>[2x]SNAMIRKYRYGAPFDTEALTEKIETAEEAFPYGEISQKEGFAFTYIMDEDDIVYGLGESNRGINKRGYCYISNCTDDPIHTEDKRSLYGAHNFIIVSGKTTFGLFFDYPSKLTFDIGYTRMDTLKVSCENADLDIYVIEGENAYDIVKQFRRVIGRSYIPPKFAFGFGQSRWGYTTKEDFRAVAKGYRENHIPIDMIYMDIDYMQDFKDFTVNEKNF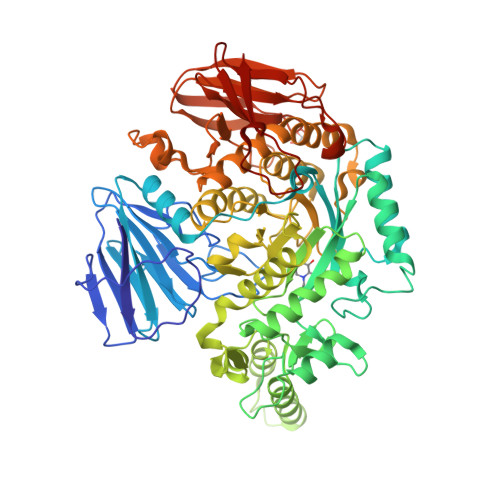PDFPEFVKEMKDQELRLIPIIDAGVKVEKGYEVYEEGVKNNYFCKREDGSDFVAAVWPGDTHFPDMLNPEARKWFGDKYRFLIDQGIEGFWNDMNEPAIFYSSEGLAEAKEFAGEFAKDTEGKIHPWAMQAKMKDIVNSPEDYKRFYHNVNGKKIRHDKVHNLFGYNMTRAAGEAFERIDPEKRFLMFSRSSYIGMHRYGGIWMGDNKSWWSHILLNLKMLPSLNMCGFMYTGADLGGFGDDTTRDLLLRFLALGVFTPLMRDHAAEGTREQECYQFENIEDFRSVINARYRLVPYLYSEYMKAALNDDMYFKPLGFVYPDDKMAIRVEDQLMLGNEIMIAPVYEQNARGRYVYLPEEMKFIKFMPDGSISEEVLEKGVHYVDVALNEVPLFIRSGKCIPVAEAAECVKDIDTENMQLIGYEGSSYTLYEDDGIHKDYDKKENYRVLTK> MSASAQQLAEELQIFGLDCEEALIEKLVELCVQYGQNEEGMVGELIAFCTSTHKVGLTSEILNSFEHEFLSKRLSKARHSTCKDSGHAGARDIVSIQELIEVEEEEEILLNSYTTPSKGSQKRAISTPETPLTKRSVSTRSPHQLLSPSSFSPSATPSQKYNSRSNRGEVVTSFGLAQGVSWSGRGGAGNISLKVLGCPEALTGSYKSMFQKLPDIREVLTCKIEELGSELKEHYKIEAFTPLLAPAQEPVTLLGQIGCDSNGKLNNKSVILEGDREHSSGAQIPVDLSELKEYSLFPGQVVIMEGINTTGRKLVATKLYEGVPLPFYQPTEEDADFEQSMVLVACGPYTTSDSITYDPLLDLIAVINHDRPDVCILFGPFLDAKHEQVENCLLTSPFEDIFKQCLRTIIEGTRSSGSHLVFVPSLRDVHHEPVYPQPPFSYSDLSREDKKQVQFVSEPCSLSINGVIFGLTSTDLLFHLGAEEISSSSGTSDRFSRILKHILTQRSYYPLYPPQEDMAIDYESFYVYAQLPVTPDVLIIPSELRYFVKDVLGCVCVNPGRLTKGQVGGTFARLYLRRPAADGAERQSPCIA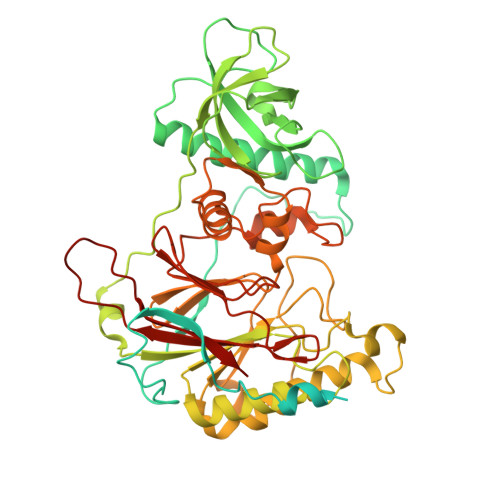VQVVRI> W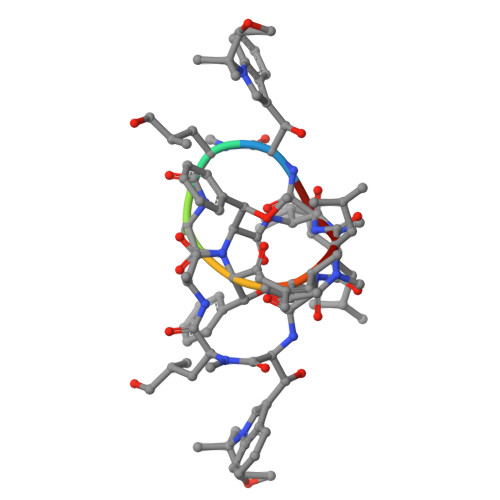LAFVLV>[2x]MPIQVLPPQLANQIAAGEVVERPASVVKELVENSLDAGATRIDIDIERGGAKLIRIRDNGCGIKKDELALALARHATSKIASLDDLEAIISLGFRGEALASISSVSRLTLTSRTAEQQEAWQAYAEGRDMNVTVKPAAHPVGTTLEVLDLFYNTPARRKFLRTEKTEFNHIDEIIRRIALARFDVTINLSHNGKIVRQYRAVPEGGQKERRLGAICGTAFLEQALAIEWQHGDLTLRGWVADPNHTTPALAEIQYCYVNGRMMRDRLINHAIRQACEDKLGADQQPAFVLYLEIDPHQVDVNVHPAKHEVRFHQSRLVHDFIYQGVLSVLQQQLETPLPLDDEPQPAPRSIPENRVAAGRNHFAEPAAREPVAPRYTPAPASGSRPAAPWPNAQPGYQKQQGEVYRQLLQTPAPMQKLKAPEPQEPALAANSQSFGRVLTIVHSDCALLERDGNISLLSLPVAERWLRQAQLTPGEAPVCAQPLLIPLR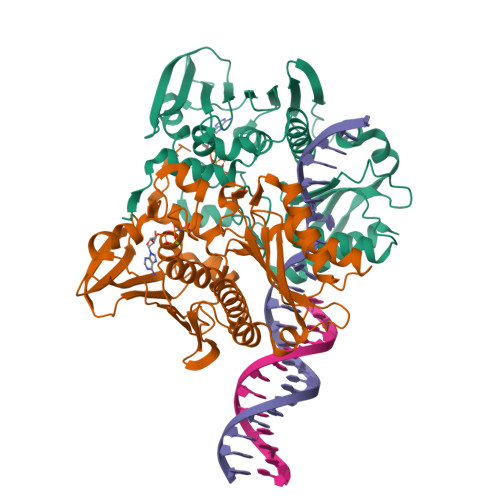LKVSAEEKSALEKAQSALAELGIDFQSDAQHVTIRAVPLPLRQQNLQILIPELIGYLAKQSVFEPGNIAQWIARNLMSEHAQWSMAQAITLLADVERLCPQLVKTPPGGLLQSVDLHPAIKALKDE>[2x]MVKLTAELIEQAAQYTNAVRDRELDLRGYKIPVIENLG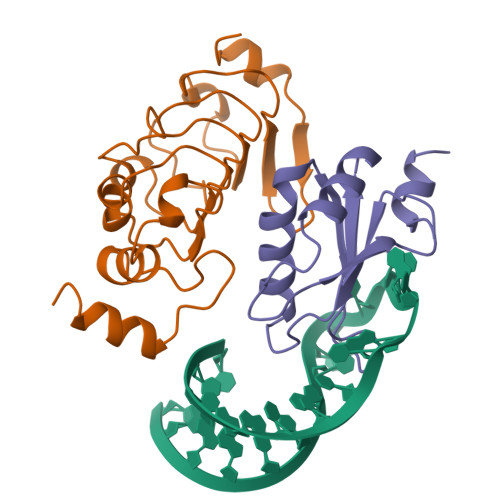ATLDQFDAIDFSDNEIRKLDGFPLLRRLKTLLVNNNRICRIGEGLDQALPDLTELILTNNSLVELGDLDPLASLKSLTYLCILRNPVTNKKHYRLYVIYKVPQVRVLDFQKVKLKERQEAEKMFKGKRGAQLAKDIAR;>[2x]MDIRPNHTIYINNMNDKIKKEELKRSLYALFSQFGHVVDIVALKTMKMRGQAFVIFKELGSSTNALRQLQGFPFYGKPMRIQYAKTDSDIISKMRG>[4x]MAVKPMLHY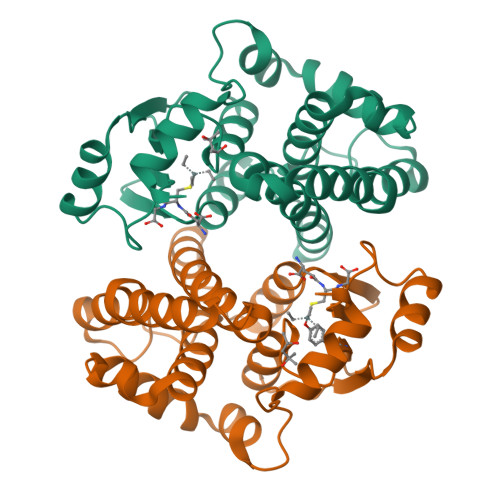FNGRGRMEPIRWLLAAAGVEFEETFIDTPEDFEKLKNDGSLMFQQVPMVEIDGMKLVQSRAILNYVAAKHNLYGKDIKERALIDMYIEGVADLNEMILLLPITPPAEKDAKIMLIKDRTTNRYLPAFEKVLKSHGEDYLVGNRLSRADIHLVELLYLVEELDPSLLTNFPLLKALKARISNLPTVKKFLQPGGARKPPGDEKSVEKSRKIFKF> MKPFNLTVAAKADLRDIALFTQRRWGKEQRNVYLKQ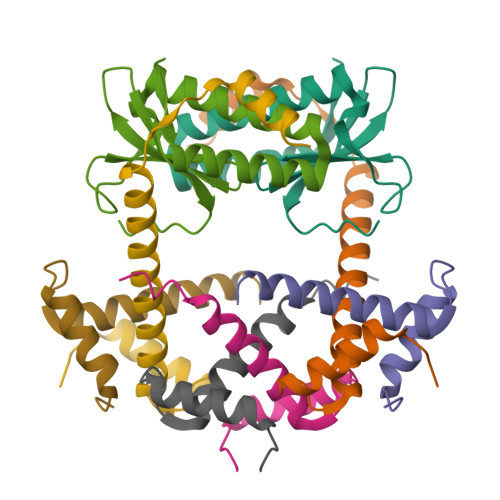FDDSFWLLAENPDIGKSCDEIREGYRKFPQGSHVIFYQQTGSQQIRVIRILHKSMDVNPIFGAHHHHHH;>[3x]MAKNTSITLGEHFDGFITSQIQSGRYGSASEVIRSALRLLENQETKLQSLRQLLIEGEQSGDADYDLDSFINELDSENIR Methylenetetrahydrofolate reductase (MTHFR) is one of the key enzymes for production of methionine, which is not only an important amino acid precursor for protein synthesis, but also the precursor of S-adenosylmethionine (AdoMet), which serves as a major methyl donor and a substrate for polyamine synthesis. MTHFR uses NAD(P)H to reduce FAD; subsequently the reduced FAD reduces methylenetetrahydrofolate (CH2-H4folate). Here, we report biochemical properties and unique crystal structures of MTHFR from T. thermophilus HB8, one of the model organisms in structural biology. We demonstrate that the Thermus MTHFR is a dimer, rather than a tetramer, so that its symmetry is perhaps more directly relevant to the dimeric mammalian MTHFR.

From sets of our experimental data, the as-purified MTHFR could be defined as a ‘heterodimer’ comprising apo- and holo- subunits, and the FAD-replete enzyme as a ‘homodimer’ formed by the two holo-subunits. In the apo-subunit, positions of the loop containing Asp109 and helix α7a are dramatically different, although the topology of the β8α8 barrel of the apo-subunit is almost identical to that of the holo-subunit. Asp109 in the apo-subunit interacts with His77, which is close to the N5-position of the isoalloxazine ring of FAD in the holo-subunit. In the holo-subunit of the as-purified MTHFR, corresponding distances were 2.83 Å, 2.68 Å and 4.37 Å, respectively, where the structure was determined from crystals at acidic pH (≈4.4). While the crystallization conditions were different, the conformational change of Thermus MTHFR is likely occurred by the ligand binding rather than by effects of hydrophobic solvent and the low pH, which we used when crystallization of the heterodimer. Similarly, the heterodimer of Thermus MTHFR may be the physiological form, since it is maximally active in catalyzing the physiological reaction. The low surface area found in the intersubunit interface of the heterodimer of Thermus MTHFR would resemble the conformation of human MTHFR without AdoMet, and the homodimer could simulate the AdoMet binding form of human MTHFR.

>[2x]MKIRDLLKARRGPLFSFEFFPPKDPEGEEALFRTLEELKAFRPAFVSITYGAMGSTRERSVAWAQRIQSLGLNPLAHLTVAGQSRKEVAEVLHRFVESGVENLLALRGDPPRGERVFRPHPEGFRYAAELVALIRERYGDRVSVGGAAYPEGHPESESLEADLRHFKAKVEAGLDFAITQLFFNNAHYFGFLERARRAGIGIPILPGIMPVTSYRQLRRFTEVCGASIPGPLLAKLERHQDDPKAVLEIGVEHAVRQVAELLEAGVEGVHFYTLNKSPATRMVLERLGLRPASGQPAKLAAALEHHHHHH Bromosporine | C17 H20 N6 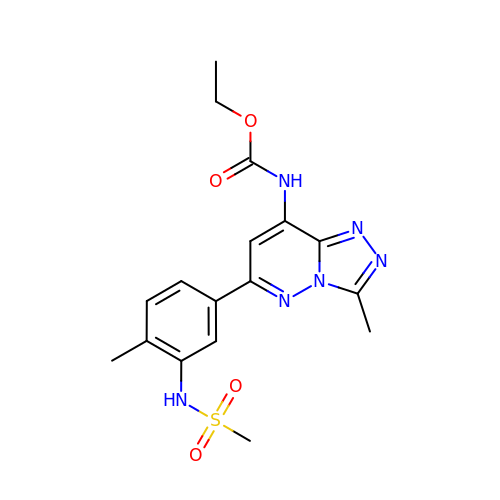O4 S | UYBRROMMFMPJAN-UHFFFAOYSA-N> MHHHHHHHAVRASEISRVYEAYPEKKATLYFLVLGFLALIVGSLFGPFQALNYGNVDAYPLLKRLLPFVQSYYQGLTLHGVLNAIVFTQLFAQAIMVYLPARELNMRPNMGLMWLSWWMAFIGLVVFALPLLANEATVLYTFYPPLKGHWAFYLGASVFVLSTWVSIYIVLDLWRRWKAANPGKVTPLVTYMAVVFWLMWFLASLGLVLEAVLFLLPWSFGLVEGVDPLVARTLFWWTGHPIAYFWLLPAYAIIYTILPKQAGGKLVSDPMARLAFLLFLLL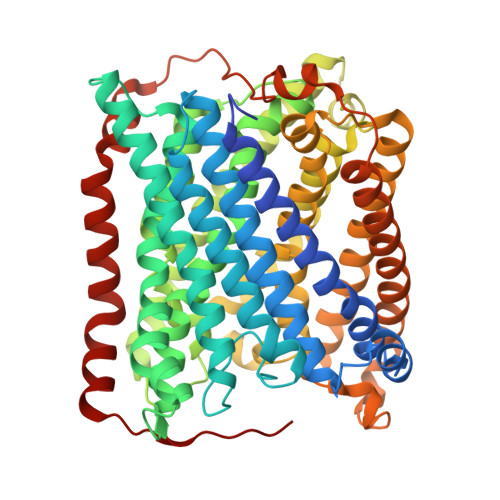STPVGFHHQFADPGIDPTWKMIHSVLTLFVAVPSLMTAFTVAASLEFAGRLRGGRGLFGWIRALPWDNPAFVAPVLGLLGFIPGGAGGIVNASFTLDYVVHNTAWVPGHFHLQVASLVTLTAMGSLYWLLPNLTGKPISDAQRRLGLAVVWLWFLGMMIMAVGLHWAGLLNVPRRAYIAQVPDAYPHAAVPMVFNVLAGIVLLVALLLFIYGLFSVLLSRERKPELAEAPLPFAEVISGPEDRRLVLAMDRIGFWFAVAAILVVLAYGPTLVQLFGHLNPVPGWRLW> SPNIEACGYSDRVMQLTLGNSTITTQEAANSVVAYGRWPEYIKDSEANPVDQPTEPDVAACRFYTLDTVTWRKESRGWWWKLPDALKDMGLFGQNMFYHYLGRAGYTVHVQCNASKFHQGALGVFAVPEMCLAGDS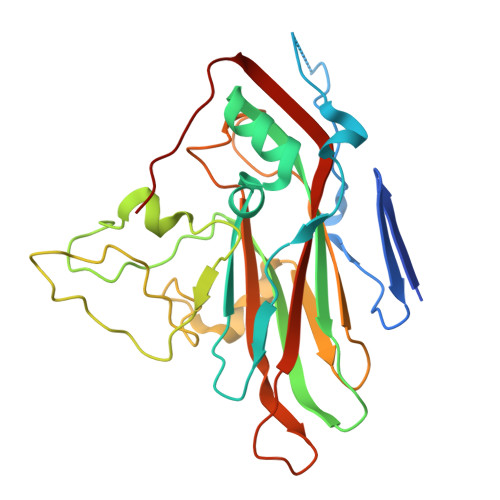TTHMFTKYENANPGEKGGEFKGSFTLDTNATNPARNFCPVDYLFGSGVLAGNAFVYPHQIINLRTNNCATLVLPYVNSLSIDSMTKHNNWGIAILPLAPLDFATESSTEIPITLTIAPMCCEFNGLRNITVPRTQ> SNADNSYKMDYPEMGLCIIINNKNFHKSTGMTSRSGTDVDAANLRETFRNLKYEVRNKNDLTREEIVELMRDVSKEDHSKRSSFVCVLLSHGEEGIIFGTNGPVDLKKITNFFRGDRCRSLTGKPKLFIIQACRGTELDCGIETASGVDDDMACHKIPVEADFLYAYSTAPGYYSWRNSKDGSWFIQS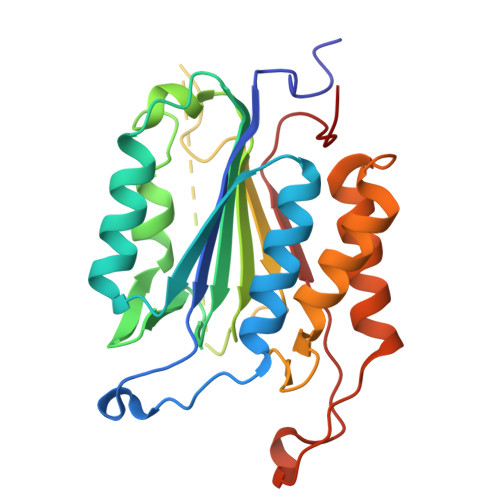LCAMLKQYADKLEFMHILTRVNRKVATEFESFSFDATFHAKKQIPCIVSMLTKELYFYH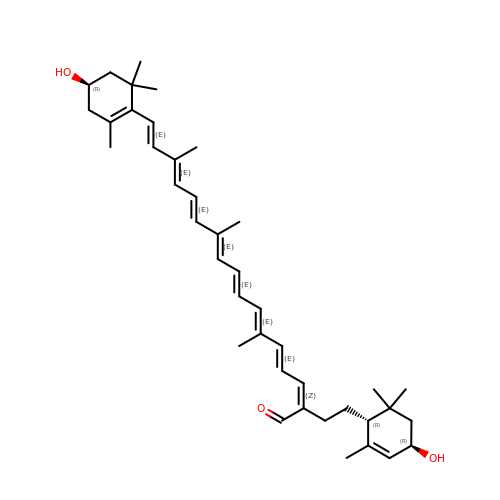(2~{Z},4~{E},6~{E},8~{E},10~{E},12~{E},14~{E},16~{E})-6,11,15-trimethyl-17-[(4~{R})-2,6,6-trimethyl-4-oxidanyl-cyclohexen-1-yl]-2-[2-[(1~{R},4~{R})-2,6,6-trimethyl-4-oxidanyl-cyclohex-2-en-1-yl]ethyl]heptadeca-2,4,6,8,10,12,14,16-octaenal | C40 H56 O3 | FJWGLEVADWWUFR-NJTXIUSISA-N> MANIDLHFHSRTSDGALTPTEVIDRAAARAPALLALTDHDCTGGLAEAAAAAARRGIPFLNGVEVSVSWGRHTVHIVGLGIDPAEPALAAGLKSIREGRLERARQMGASLEAAGIAGCFDGAMRWCDNPEMISRTHFARHLVDSGAVKDMRTVFRKYLTPGKPGYVSHQWASLEDAVGWIVGAGGMAVIAHPGRYDMGRTLIERLILDFQAAGGQ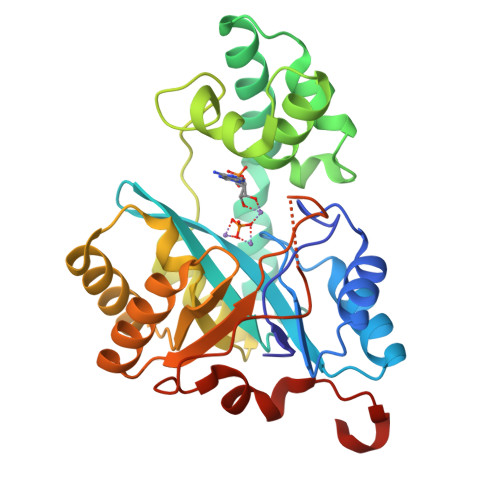GIEVASGSHSLDDMHKFALHADRHGLYASSGSDFHAPGEGGRDVGHTEDLPPICRPIWRELEARILRPADAENLYFQ> MKNVGFIGWRGMVGSVLMDRMSQENDFEN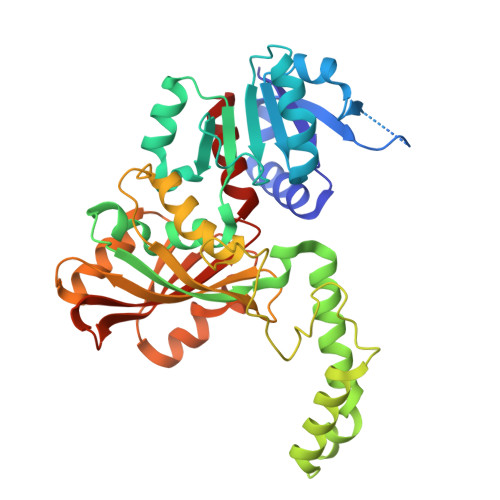LNPVFFTTSQAGQKAPVFGGKDAGDLKSAFDIEELKKLDIIVTCQGGDYTNEVYPKLKATGWDGYWVDAASALRMKDDAIIVLDPVNQHVISEGLKKGIKTFVGGNCTVSLMLMAIGGLFEKDLVEWISVATYQAASGAGAKNMRELLSQMGLLEQAVSSELKDPASSILDIERKVTAKMRADNFPTDNFGAALGGSLIPWIDKLLPETGQTKEEWKGYAETNKILGLSDNPIPVDGLCVKIGALRCHSQAFTIKLKKDLPLEEIEQIIASHNEWVKVIPNDKEITLRELTPAKVTGTLSVPVGRLRKLAMGPEYLAAFTVGDQLLWGAAEPVRRILKQLVA>[8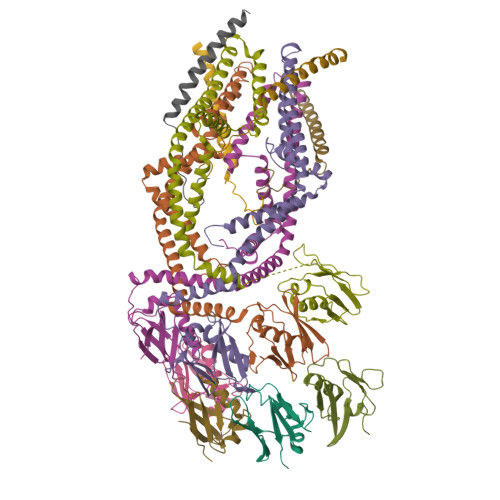x]MAAAAGRSLLLLLSSRGGGGGGAGGCGALTAGCFPGLGVSRHRQQQHHRTVHQRIASWQNLGAVYCSTVVPSDDVTVVYQNGLPVISVRLPSRRERCQFTLKPISDSVGVFLRQLQEEDRGIDRVAIYSPDGVRVAASTGIDLLLLDDFKLVINDLTYHVRPPKRDLLSHENAATLNDVKTLVQQLYTTLCIEQHQLNKERELIERLEDLKEQLAPLEKVRIEISRKAEKRTTLVLWGGLAYMATQFGILARLTWWEYSWDIMEPVTYFITYGSAMAMYAYFVMTRQEYVYPEARDRQYLLFFHKGAKKSRFDLEKYNQLKDAIAQAEMDLKRLRDPLQVHLPLRQIGEKD;>MASGAARWLVLAPVRSGALRSGPSLRKDGDVSAAWSGSGRSLVPSRSVIVTRSGAILPKPVKMSFGLLRVFSIVIPFLYVGTLISKNFAALLEEHDIFVPEDDDDDD[4x]> GCACUAGAUCGGAUG;> ATCCGATGGATCATACGGTCGGAGG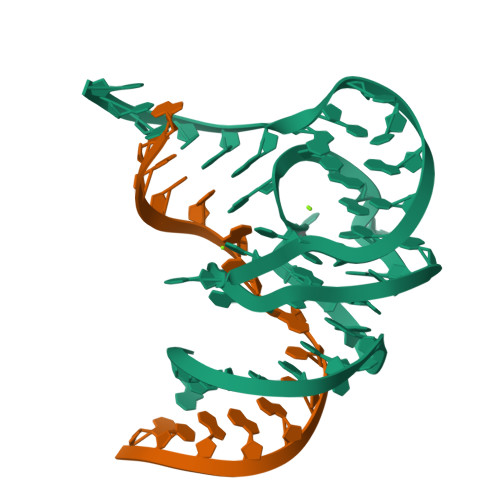GGTTTGCCGTTTAAGTGCC>[2x]SDLIVKDNALMNASYNLALVEQRLILLAIIEARETGKGINANDPLTVHASSYINQFNVERHTAYQALKDACKDLFARQF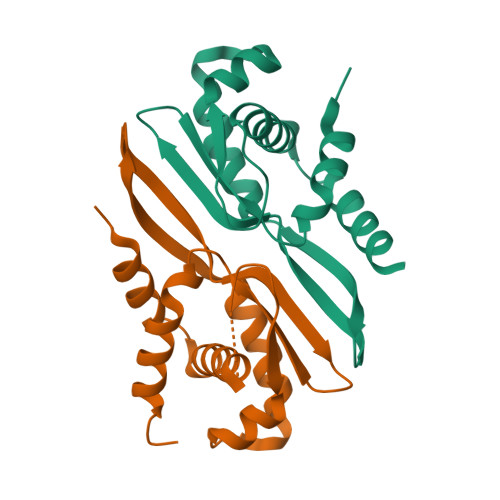SYQEKRERGRINITSRWVSQIGYMDDTATVEIIFAPAVVPLITRLEEQFTQYDIEQ>GPLGSSQIPASEQETLVRPKPLLLKLLKSVGAQKDTYTMKEVLFYLGQYIMTKRLYDAAQQHIVYCSNDLLGDL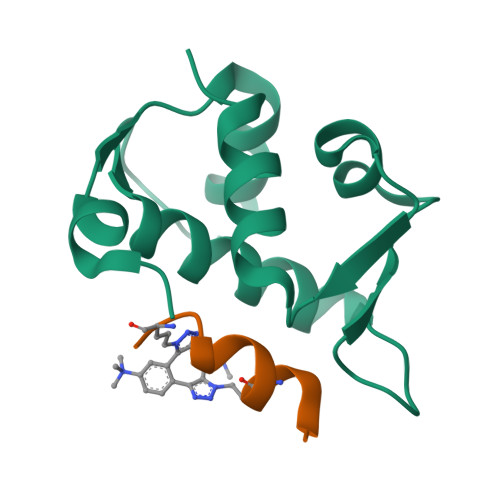FGVPSFSVKEHRKIYTMIYRNLV[2x];>[2x]XLTFAEYWAQLASX>[4x]MKLAVYSTKQYDKKYLQQVNESFGFELEFFDFLLTEKTAKTANGCEAVCIFVNDDGSRPVLEELKKHGVKYIALRCAGFNNVDLDAAKELGLKVVRVPAYDPEAVAEHAIGM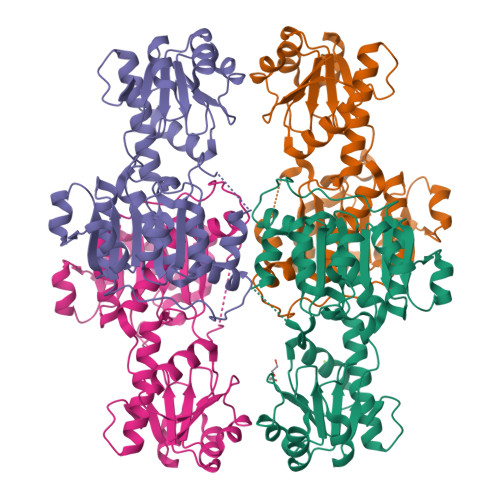MMTLNRRIHRAYQRTRDANFSLEGLTGFTMYGKTAGVIGTGKIGVAMLRILKGFGMRLLAFDPYPSAAALELGVEYVDLPTLFSESDVISLHCPLTPENYHLLNEAAFDQMKNGVMIVNTSRGALIDSQAAIEALKNQKIGSLGMDVYENERDLFFEDKSNDVIQDDVFRRLSACHNVLFTGHQAFLTAEALTSISQTTLQNLSNLEKGETCPNELV> GPLSVAPEMDIMDYCKKEWRGNTQKATCMKMGYEEVSQKFTSIRRVRGDNYCALRATLFQAMSQAVGLPPWLQDPELMLLPEKLISKYNWIKQWKLGLKFDGKNEDLVDKIKESLTLLRKKWAGLAEMRTAEARQIACDELFTNEAEEYSLYEAVKFLMLNRAIELYNDKEKGKEVPFFSVLLFARDTSNDPGQLLRNHLNQVRHTGGLEQVEMFLLAYAVRHTIQVYRLSKYNTEEFITVYPTDPPKDWPVVTLIAEDDRHYNIPVR

OTULIN (OTU family deubiquitinase with linear Ub specificity, also known as FAM105B or Gumby) is the only DUB known to specifically cleave M1 linkages (Keusekotten et al, 2013; Rivkin et al, 2013). The deubiquitinase OTULIN removes methionine‐1 (M1)‐linked polyubiquitin signals conjugated by the linear ubiquitin chain assembly complex (LUBAC) and is critical for preventing TNF‐driven inflammation in OTULIN‐related autoinflammatory syndrome (ORAS). Several studies have shown that OTULIN binds directly to the LUBAC subunit HOIP (Elliott et al, 2014; Schaeffer et al, 2014; Takiuchi et al, 2014). OTULIN‐related autoinflammatory syndrome (ORAS) (also known as otulipenia or autoinflammation, panniculitis and dermatosis syndrome (AIPDS); OMIM ID: 617099) is a potentially fatal, TNF‐driven autoinflammatory disease characterised by sterile systemic inflammation, recurrent high fevers, panniculitis, diarrhoea, arthritis and general failure to thrive (Damgaard et al, 2016; Zhou et al, 2016).

Gly281 is evolutionarily conserved and located in a loop between helices α11 and α12 (Fig EV1A; Keusekotten et al, 2013). Together with His282 and Thr283, Gly281 forms part of the Ub‐binding site and makes direct contacts to the proximal Ub of M1‐linked diUb bound across the active site (Figs 2A, centre panel and EV1A; Keusekotten et al, 2013). To understand the pathogenicity of the Gly281Arg mutation on OTULIN, we crystallised OTULIN's catalytic domain (OTULINcat, aa 80–352) containing the Gly281Arg ORAS mutation (OTULINcatG281R) and determined its structure to 1.8 Å resolution. Overall, the structure showed that OTULINcatG281R adopted an OTU fold similar to OTULINcatWT (Keusekotten et al, 2013) without any major perturbations. However, comparing the structure of OTULINcatG281R with the previously solved structure of OTULINcat in complex with M1‐linked diUb (Keusekotten et al, 2013) showed that the Gly281Arg mutation partly unfolds the substrate‐binding site. The introduced Arg side chain can no longer fit into the narrow pocket between helices α3 and α9 thereby flipping the Gly281‐containing loop out of its normal binding groove (Keusekotten et al, 2013). In the mutant protein, the loop has increased flexibility, as represented by the high crystallographic B‐factor distribution across the loop compared to other regions within the OTU domain (Fig EV1B) and also evidenced by lack of interpretable electron density for the side chains of Val280, mutated Arg281 and His282 (Fig EV1C). The new conformation of the Gly281‐containing loop indicated that His282 and Thr283 would clash with M1‐linked diUb at the binding site and prevent substrate binding. OTULING281R was ~20‐200 times less active towards M1‐linked tetraUb compared with OTULINWT. In addition to reduced Ub binding and activity, the Gly281Arg mutation caused a considerable intrinsic destabilisation of OTULIN.> MTTYGSSVPEQQITAYLSRIQRGGYIQPFGCMIAVDESSFRIIGYSENAREMLGIMPQSVPTLEKPEILAMGTDVRSLFTSSSSILLERAFVAREITLLNPVWIHSKNTGKPFYAILHRIDVGVVIDLEPARTEDPALSIAGAVQSQKLAVRAISQLQALPGGDIKLLCDTVVESVRDLTGYDRVMVYKFHEDEHGEVVAESKRDDLEPYIGLHYPATDIPQASRFLFKQNRVRMIVDCNATPVLVVQDDRLTQSMCLVGSTLRAPHGCHSQYMANMGSIASLAMAVIINGNEDDGSNVASGRSSMRLWGLVVCHHTSSRCIPFPLRYACEFLMQAFGLQLNMELQLALQMSEKRVLRTQTLLCDMLLRDSPAGIVTQSPSIMDLVKCDGAAFLYHGKYYPLGVAPSEVQIKDVVEWLLANHADSTGLSTDSLGDAGYPGAAALGDAVCGMAVAYITKRDFLFWFRSHTAKEIKWGGAKHHPEDKDDGQRMHPRSSFQAFLEVVKSRSQPWETAEMDAIHSLQLILRDSFKESEAASLHHHHHH;> MTTYGSSVPEQQITAYLSRIQRGGYIQPFGCMIAVDESSFRIIGYSENAREMLGIMPQSVPTLEKPEILAMGTDVRSLFTSSSSILLERAFVAREITLLNPVWIHSKNTGKPFYAILHRIDVGVVIDLEPARTEDPALSIAGAVQSQKLAVRAISQLQALPGGDIKLLCDTVVESVRDLTGYDRVMVYKFHEDEHGEVVAESKRDDLEPYIGLHYPATDIPQASRFLFKQNRVRMIVDCNATPVLVVQDDRLTQSMCLVGSTLRAPHGCHSQYMANMGSIASLAMAVIINGNEDDGSNVASGRSSMRLWGLVVCHHTSSRCIPFPLRYACEFLMQAFGLQLNMELQLALQMSEKRVLRT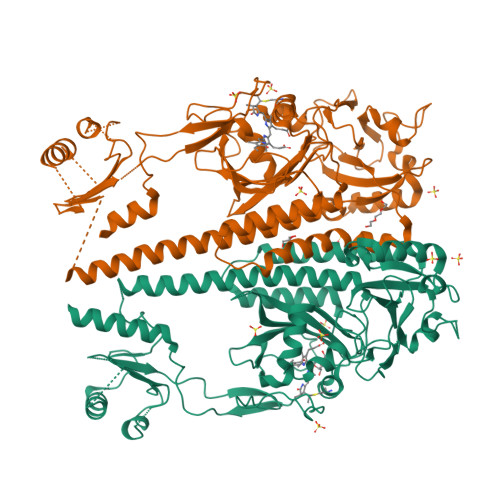QTLLCDMLLRDSPAGIVTQSPSIMDLVKCDGAAFLYHGKYYPLGVAPSXXXXXXXXXXXXXNHADSTGLSTDSLGDAXXXXXXALGDAVCGMAVAYITKRDFLFWFRSHTAKEIKWGGAKHHPEDKDDGQRMHPRSSFQAFLEVVKSRSQPWETAEMDAIHSLQLILRDSFKESEAASLHHHHHH> MSKPQPIAAANWKCNGSQQSLSELIDLFNSTSINHDVQCVVASTFVHLAMTKERLSHPKFVIAAQNAGNADALASLKDFGVNWIVLGHSERRAYYGETNEIVADKVAAAVASGFMVIACIGETLQERESGRTA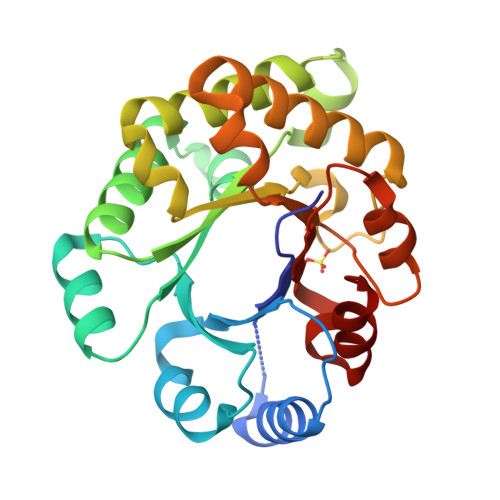VVVLTQIAAIAKKLKKADWAKVVIAYEPVWAIGTGKVATPQQAQEAHALIRSWVSSKIGADVAGELRILYGGSVNGKNARTLYQQRDVNGFLVGGASLKPEFVDIIKATQ>MVSSDRPVSLEDEVSHSMKEMIGGCCVCSDERGWAENPLVYCDGHGCSVAVHQACYGIVQVPTGPWFCRKCESQERAARVRCELCPHKDGALKRTDNGGWAHVVCALYIPEVQFANVSTMEPIVLQSVPHDRYNKTCYICDEQGRESKAATGACMTCNKHGCRQAFHVTCAQFA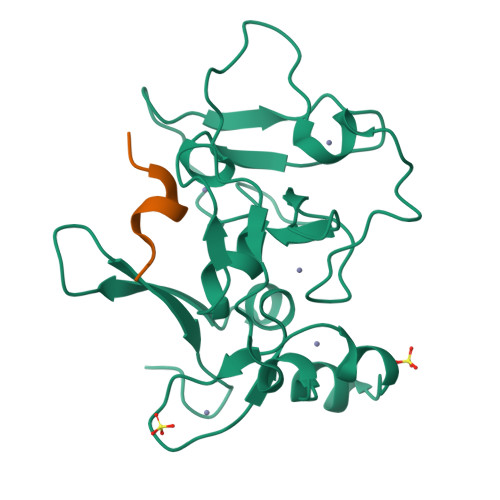GLLCEEEGNGADNVQYCGYCKYHFSKLKKSKRGS[2x];>[2x]QLATKAARKSA> MTLNTVALELVPSNLDLGTAHALAELQKVRKLAVDAGLDGRIRHIMIPGMIEEDDGRPVEMKPKLDVLDYWELVQRELPDVRGLCTQVTSFLGERSLRRRLTALIQHGFEGIAFVGVPRTMTDGEGAGVAPTDALSTFSHLVKHRGVILIPTRDDELSRFGFKCKEGATFGMT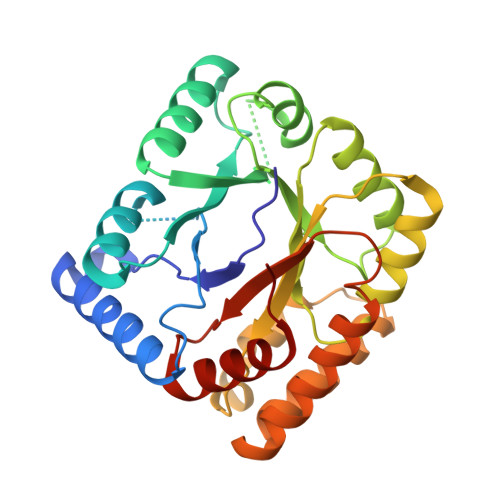QLLYSDAIVNFLTEFSRNTDHRPEILLSFGFVPKMESEVGLIDWLIQDPDNGAVATEQQFVRRLAASEPAQKRAQMLDLYKRVIDGVIDLGFPVSLHFEAPYGVSAPAFETFAAMLDYWAPDR Among families of proteins involved in signal transduction, phospholipase C (PLC) enzymes that generate second messengers from phosphatidylinositol 4,5-bisphosphate (PIP2) incorporate a number of different protein modules. PLCγ enzymes (PLCγ1 and PLCγ2), for example, contain eight domains, four of which are unique to this PLC family (Bunney and Katan, 2011; Suh et al., 2008). The PLCγ ‘specific array’ of domains (γSA), comprising a “split” PH (spPH) domain flanking two tandem SH2 domains and an SH3 domain, is inserted between the two halves (X and Y) of the TIM-barrel catalytic domain (Bunney and Katan, 2011). We demonstrate that among four domains present in the γSA, the cSH2 domain and its C-terminal linker provide a focus for most interdomain interactions both within the γSA and between the γSA and the PLC-core.

In addition, we solved the structure of the tandem nSH2-cSH2 pair by X-ray crystallography. Based on the determination of the crystal structure of the PLCγ1 tandem nSH2-cSH2 domains in nonliganded form (left), suggesting that these SH2 domains might possess limited intramolecular flexibility with respect to each other, we directly tested this hypothesis. We recorded 15N relaxation data on the tandem and isolated SH2 domains. The error-weighted mean 15N R2/R1 ratio (24.0 ± 0.7) obtained for 68 resolved cross peaks, is substantially larger than would be expected for the isolated domains. The corresponding derived isotropic rotational correlation time (15.5 ± 0.6 ns; TENSOR2) is closer to that predicted from the X-ray crystal structure using hydrodynamic modeling (18.6 ns; HYDRONMR) applied to residues 549–772 of the tandem than to the prediction for the isolated domains (7.4 and 8 ns) (right). This suggests that the tandem construct tumbles as a more-or-less rigid entity in solution. Restraints are imposed on the cSH2 domain by an apparently inflexible linker to the nSH2 domain. Indeed the two SH2 domains could be thought of as forming a single supramodule as defined by the NMR-derived rotational correlation time. Intriguingly, some less defined density is also observed in the peptide-binding groove for cystals obtained for the nonphosphorylated tandem nSH2-cSH2 protein, suggesting that in the absence of other interactions that might take place within the full-length PLCγ1 (see further) the region of the cSH2-SH3 linker has certain affinity in cis for the pY peptide binding site even in the absence of Y783 phosphorylation. Although the structure of the cSH2 domain is not affected upon pY783 binding, a further, more detailed comparison of the crystal structure of the phosphorylated nSH2-cSH2 protein with the nonphospho (apo) construct in the same crystal form shows general similarity with some subtle differences in angle and distance between the domains (not shown).

> HSNEKWFHGKLGAGRDGRHIAERLLTEYCIETGAPDGSFLVRESETFVGDYTLSFWRNGKVQHCRIHSRQDAGTPKFFLTDNLVFDSLYDLITHYQQVPLRCNEFEMRLSEPVPQTNAHESKEWYHASLTRAQAEHMLMRVPRDGAFLVRKRNEPNSYAISFRAEGKIKHCRVQQEGQTVMLGNSEFDSLVDLISYYEKHPLYRKMKLRYPINEEALEKIGTAEPDYGALYEGRNPGFYVEANPMP>GMSVVDPSLIERIIRDDVRAMGAYHVPDSHGLVKLDAMENPYRLPPALRSELAARLGEVALNRYPVPSSEALRAKLKEVMQVPAGMEVLLGNGSDEIISMLALAAARPGAKVMAPVPGFVMYAMSAQFAGLEFVGVPLRADFTLDRGAMLAAMAEHQPAIVYLAYPNNPTGNLFDAADMEAIVRAAQGSVCRSLVVVDEAYQPFAQESWMSRLTDFGNLLVMRTVSKLGLAGIRLGYVAGDPQWLEQLDKVRPPYNVNVLTEATALFA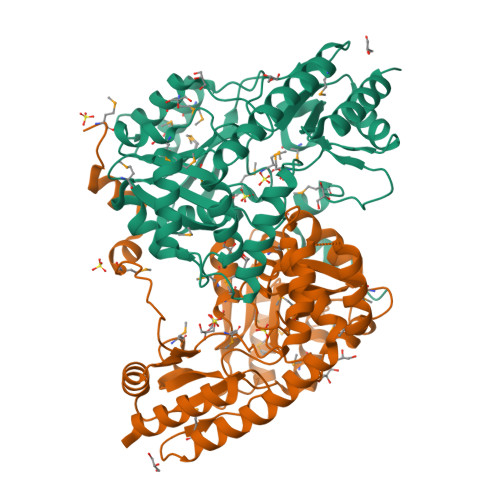LEHVAVLDEQAAQLRAERSRVAEGMAAHGGVTVFPSAANFLLARVPDAAQTFDRLLARKVLIKNVSKMHPLLANCLRVTVSTPEENAQFLEAFAASLQD[2x]> GAASPKQIQMWINNVA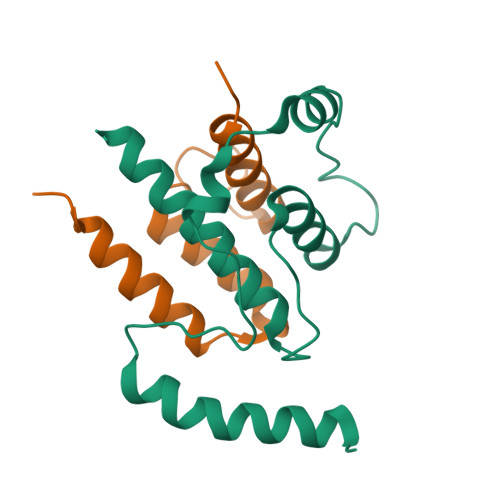EIRKTKQPHSVSYTKPMPEIDELMQEWPQEIEEILQHLKIPSEELDFNLSDFCKLACAILDIPVHDQPNESNVIESLHVLFTLYSEFKSNQHFQQNKNDG;> GAASDEFASEKVRLAQLTNKCNNNDLDYYIKESGDILGVTDKVKNKHDAKAILRYVLEELINFKKLNN> KEVCYERLGCFSDDSPWSGITERPLHILPWSPKDVNTRFLLYTNENPNNFQEVAADSSSISGSNFKTNRKTRFIIHGFIDKGEENWLANVCKNLFKVESVNCICVDWKGGSRTGYTQASQNIRIVGAEVAYFVEFLQSAFGYSPSNVHVIGHSLGAHAAGEAGRRTNGTIGRITGLDPAEPCFQGTPELVRLDPSDAKF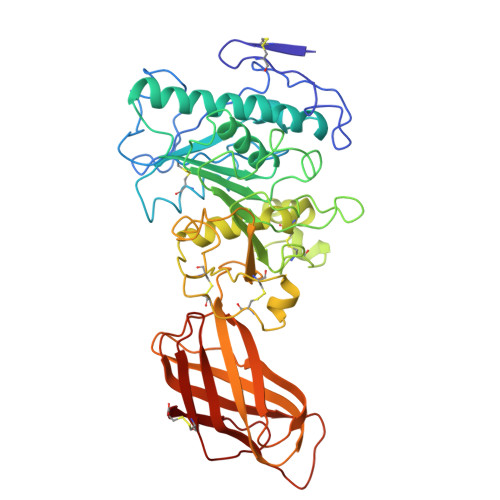VDVIHTDGAPIVPNLGFGMSQVVGHLDFFPNGGVEMPGCKKNILSQIVDIDGIWEGTRDFAACNHLRSYKYYTDSIVNPDGFAGFPCASYNVFTANKCFPCPSGGCPQMGHYADRYPGKTNDVGQKFYLDTGDASNFARWRYKVSVTLSGKKVTGHILVSLFGNKGNSKQYEIFKGTLKPDSTHSNEFDSDVDVGDLQMVKFIWYNNVINPTLPRVGASKIIVETNVGKQFNFCSPETVREEVLLTLTPC>[3x]MWPSAKFIDGRVAFSRMPAERELDEVARDFDAVVVLVEDYELPYSL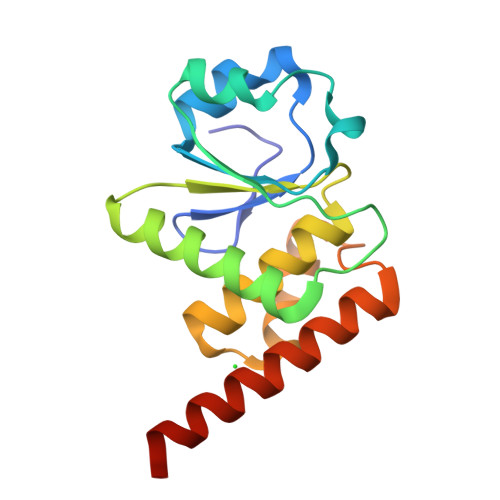DEWEKRGVEVLHGPIPDFTAPSVEQLLEILRWIEERVREGKKVLIHCMAGLGRSGTVGVAWLMYSRGLSLREALMEVRRKRPGAVETQEQMEVLKELEERIKLAAALEHHHHHH>[2x]MSLAKDVTIIYTNDLHAHVEPYKVPWIADGKRDIGGWANITTLVKQEKAKNKATWFFDAGDYFTGPYISSLTKGKAIIDIMNTMPFDAVTIGNHEFDHGWDNTLLQLSQAKFPIVQGNIFYQNSSKSFWDKPYTIIEKDGVKIGVIGLHGVFAFNDTVSAATRVGIEARDEIKWLQRYIDELKGKVDLTVALIHEGVPARQSSMGGTDVRRALDKDIQTASQVKGLDILITGHAHVGTPEPIKVGNTLILSTDSGGIDVGKLVLDYKEKPHNFTVKNFELKTIYADEWKPDQQTKQVIDGWNKKLDEVVQQTVAQSPVELKRAYGESASLGNLAADALLAAAGKNTQLALTNSGGIRNEIPAGAITMGGVISTFPFP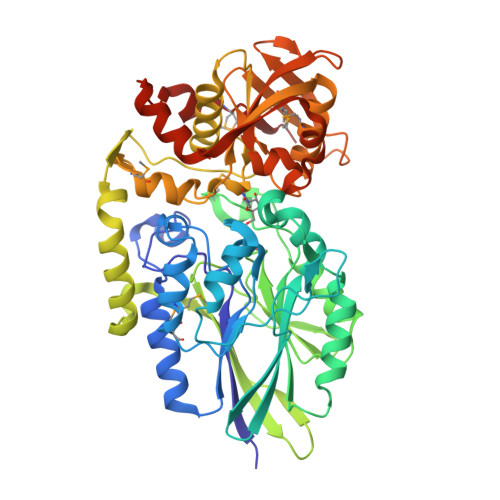NELVTMELTGKQLRSLMEHGASLSNGVLQVSKGLEMKYDSSKPVGQRVITLTLNGKPIEDATVYHIATQSFLADGGDGFTAFTEGKARNITGGYYVYHAVVDYFKAGNTITDEQLNGMRVKDIKEGHHHHHH>GSPGISGGGGGSASPNSPKDNTWIQA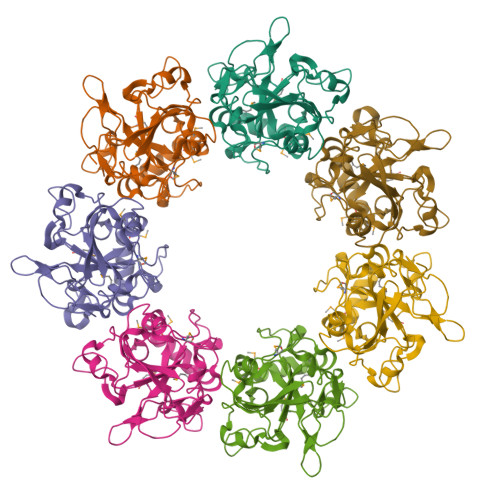ASLTWLMDMSSLLYQLISTRIPSFASPNGLHMREQTIDSNTGQIQIDNEHRLLRWDRRPPNDIFLNGFIPRVTNQNLSPVEDTHLLNYLRTNSPSIFVSTTRARYNNLGLEITPWTPHSANNNIIYRYEIFAPGGIDINASFSRNHNPFPNEDQITFPGGIRPEFIRSTYEYHNGEIVRIWINPNFINPSTLNDVSGPSNISKVFWHENHSEGNNMDSKGFILDLDYNQDFDMFAPNGEIPNNNLLNNNSLNVIQNSEYQIKNKK[14x]>[3x]MKIDPIRETTDEARALARQLLEAARHASLGTLDPETGVPLVTRIALQTDADGVPLALLAGLAAHARALAVDPRAGLLIAAEAAKGDAMTHARLSILGRAVPAEPDENRRARWLERDPKAKVYLDLPDFRFWRIEPVSGLLNAGFGQAFKLTASDMLKPPAE

Within the opp operon is a gene (pden_1323) annotated by the National Center for Biotechnology Information (NCBI) as a pyridoxamine 5′-phosphate (PMP) oxidase-related FMN-binding protein. PMP oxidases belong to the same superfamily as HugZ-like HOs, which motivated investigation of Pden_1323 as a HO. Here, we show that Pden_1323 is an unusual HO that shows specificity for the degradation of c-type heme instead of b-type heme, differentiating it from all previously characterized HOs. Activity assays of Pden_1323 with the hemopeptide substrate microperoxidase-11 (MP-11) show c-type heme degradation to free iron, CO, and a peptide-linked β- and/or δ-biliverdin.

The X-ray crystal structure of Pden_1323 was solved and found to form a dimeric split β-barrel similar to HugZ. However, comparison of the active sites of Pden_1323 and HugZ shows stark differences. While the two residues of HugZ that form salt bridging interactions with the carboxylates of heme, His163 and Arg166, are conserved in the structure of Pden_1323 (His64 and Arg92), the entire N-terminal α/β domain of HugZ is not present in the structure of Pden_1323 (25). Furthermore, the C-terminal loop that contains the coordinating heme ligand is not found in the Pden_1323 structure. Taken together, the lack of the N-terminal domain and C-terminal loop indicates that the presumed active site of Pden_1323 is only partially formed, which provides a rationale for Pden_1323's lack of HO activity with free heme. Given these structural characteristics, combined with the fact that pden_1323 is found within a gene cluster that is likely involved in the transport of both heme and peptides, it was reasoned that the substrate of Pden_1323 may instead be a c-type hemopeptide. The inability of Pden_1323 to cleave full-length cytochrome c shows that the peptide linkage must be small enough so that the porphyrin macrocycle is not buried and is able to access the active site, while the cleavage of hemin at high imidazole concentration indicates that the histidine lower axial ligand (rather than the c-type thioether linkages or the peptide sequence) is the crucial factor enabling catalysis. This suggests that Pden_1323 may bind a range of hemopeptide substrates in a way that creates a HugZ-like active site, with the histidine residue provided by the peptide substrate coordinating and activating the heme iron. The structural comparison of HugZ and Pden_1323 suggests that the change in substrate specificity from free heme b to a c-type hemopeptide involves the loss of the C-terminal loop containing the coordinating heme ligand and an opening of the active site to accommodate the larger substrate via loss of the N-terminal α/β domain. In contrast, HupZ lacks both the N-terminal α/β domain and C-terminal loop and thus more closely resembles Pden_1323 (36).> NLYQFKNMIQCTVPSRSWADFADYGCYCGKGGSGTPVDDLDRCCQTHDNCYNEAENISGCRPKFKTYSYECTQGTLTCKGDNNACAASVCD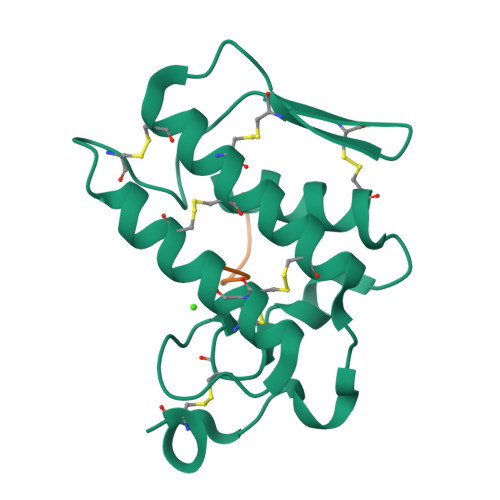CDRLAAICFAGAPYNDANYNIDLKARCN;> VGGVVIA> MFAKQIDIHWQKMKGIKFLHWLLGTVLLWVSLSTPALAIPALDYNPWEAIQLPTTATILDMSFIDRHHGWLVGVNATLMETRDGGQTWEPRTLVLDHSDYRFNSVSFQGNEGWIVGEPPIMLHTTDGGQSWSQIPLDPKLPGSPRLIKALGNGSAEMITNVGAIYRTKDSGKNWQALVQEAIGVMRNLNRSPSGEYVAVSSRGSFYSTWEPGQTAWEPHNRTTSRRLHNMGFTPDGRLWMIVNGGKIAFS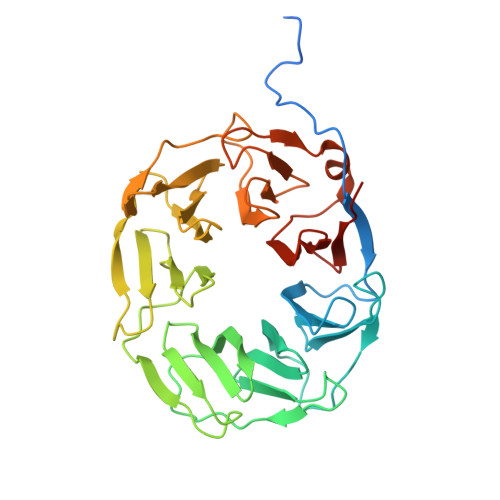DPDNSENWGELLSPLRRNSVGFLDLAYRTPNEVWLAGGAGALLCSQDGGQTWQQDVDVKKVPSNFYKILFFSPDQGFILGQKGILLRYVTDLTAAPA> KYEYVELAKASLTSAQPQHFYAVVIDATFPYKTNQERYICSLKIVDPTLYLKQQKGAGDASDYATLVLYAKRFEDLPIIHRAGDIIRVHRATLRLYNGQRQFNANVFYSSSWALFSTDKRSVTQEINNQDAVSDTTPFSFSSKHATIEKNEISILQNLRKWANQYFSSYSVISSDMYTALNKAQAQKGDFDVVAKILQVHELDEYTNELKLKDASGQVFYTLSLKLKFPHVRTGEVVRIRSATYDETSTQKKVLILSHYSNIITFIQSSKLAKELRAKIQDDHSVEVASLKKNVSLNAVVLTEVDKKHA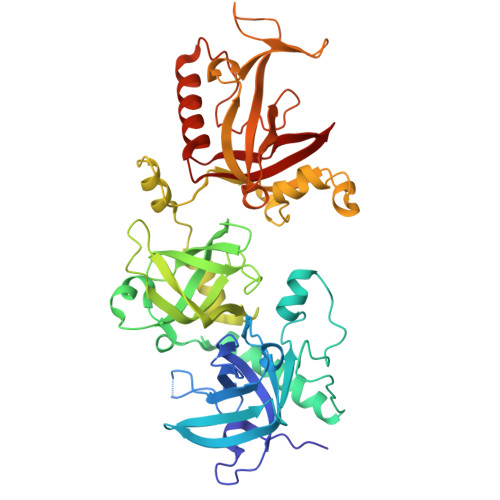ALPSTSLQDLFHHADSDKELQAQDTFRTQFYVTKIEPSDVKEWVKGYDRKTKKSSSLKGASGKGDNIFQVQFLVKDASTQLNNNTYRVLLYTQDGLGANFFNVKADNLHKNADARKKLEDSAELLTKFNSYVDAVVERRNGFYLIKDTKLIY>AADTAPADSLYSRMGGEAAVEKAVDVFYERIVADPQLAPFFANVDMKKQRRKQVAFMTYVFG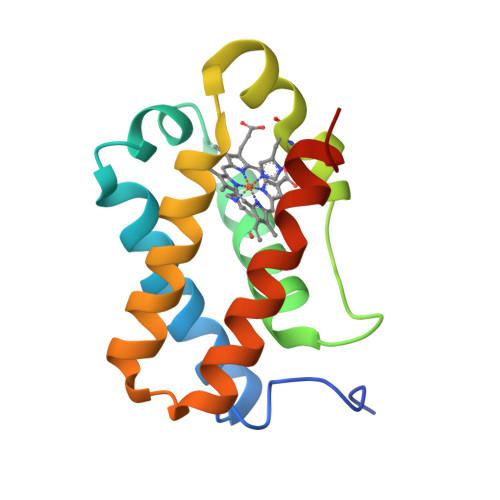GSGAYEGRDLGASHRRLIREQGMNHHHFDLVAAHLDSTLQELGVAQELKAEAMAIVASARPLIFGTGEAGAAN[2x]>[2x]MVTGGMASKWDQKGMDIAYEEAALGYKEGGVPIGGCLINNKDGSVLGRGHNMRFQKGSATLH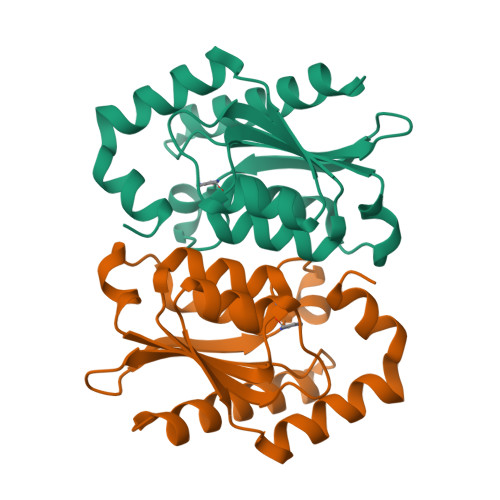GEISTLENCGRLEGKVYKDTTLYTTLSPCDMCTGAIIMYGIPRCVVGENVNFKSKGEKYLQTRGHEVVVVDDERCKKIMKQFIDERPQDWFEDIGE>[2x]MTATVTERTVEMYPLKSRLLEVVNVRRITPRMVRVDLGGSDIAGLRSDNFADHVKLWFPNPETGEHVLPVVEDDRCLNFRAPGVIYR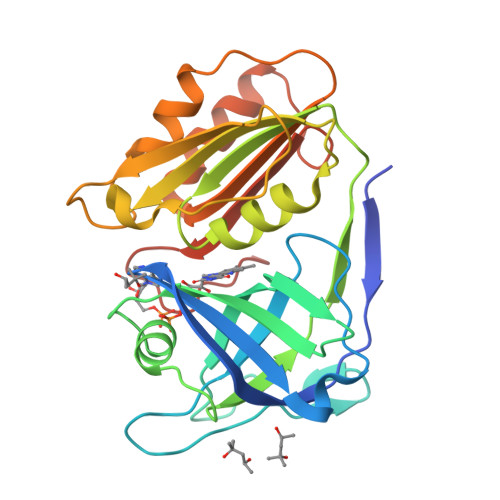DYTVRRFDAKARLLTIDFVVHDNGPGGRWAATAQPGDRLGVLGPRGTVYYPEADHYVLLADETALPAAARRIEELPRDASVTAFFEVADAAEEQELDAPEGAEITWLHRNGAAPGTTDLLLRALEQTEFPKGRVFVWAGGEADALKPIRRLLKERGLVRGRDFEVDGYWRRGVSNLDHHAADDDDE> GAGAGAMSSDTHGTDLADGDVLVTGAAGFIGSHLVTELRNSGRNVVAVDRRPLPDDLESTSPPFTGSLREIRGDLNSLNLVDCLKNISTVFHLAALPGVRPSWTQFPEYLRCNVLATQRLMEACVQAGVERVVVASSSSVYGGADGVMSEDDLPRPLSPYGVTKLAAERLALAFAARGDAELSVGALRFFTVYGPGQRPDMFISRLIRATLRGEPVEIYGDGTQLRDFTHVSDVVRALMLTASVRDRGSAVLNIGTGSAVSVNEVVSMTAELTGLRPCTAYGSARIGDVRSTTADVRQAQSVLGFTARTGL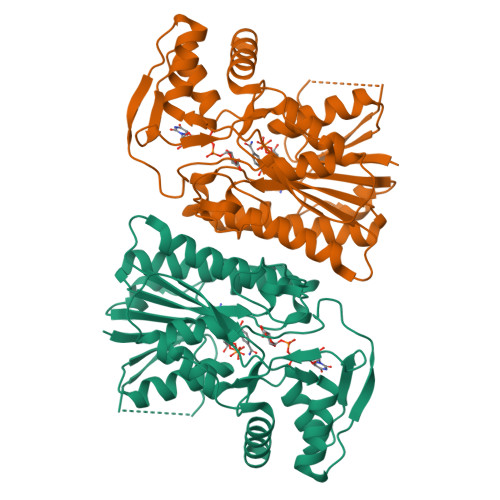REGLATQIEWTRRSLSGAEQDTVPVGGSSVSVPRL> GPLGSPEFPGAFRTQKPSLNTVNVVGSSMGSGGVFTIDGKIKCVTAAHVLTGNSARVSGVGFNQMLDFDVKGDFAIADCPNWQGVAPKAQFCEDGWTGRAYWLTSSGVEPGVIGNGFAFCFTACGDAGSPVITEAGELVGVHTGSNKQGGGIVTRPSGQFCNVKPI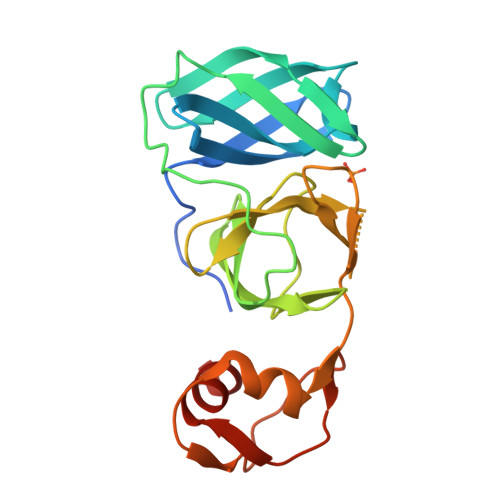KLSELSEFFAGPKVPLGDVKIGSHIIKDTCEVPSDLCALLAAKPELE>MDLSGKMVKQVEILSDGIVFYEIFRYRLY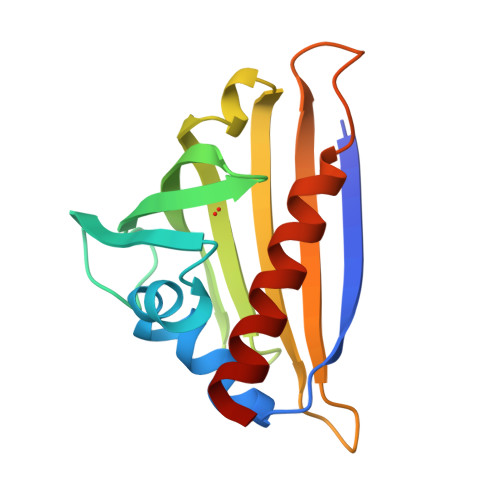LISEMSPVNIQGVDLLEGNWGTVGSVIFFKYTIDGKEKTAKDIVEAIDEETKSVTFKIVEGDLMELYKTFIIIVQVDTKGEHNSVTWTFHYEKLKEDVEEPNTLMNFCIEITKDIETYHLK[4x]>GHMSKSDYIQNMFQTKSFVDRYKYTEKLTGLYAQTLVDYSGVANTSQKPLIVLDNACGIGAVSSVLNHTLQDEAKKTWKLTCGDLSEGMLETTKRRLQDEGWVNAETKIVNALDTGLPDGHYTHVFVAFGFQSFPDANAALKECFRILASGGILASSTWQNFNWIPIMKAAIETIPGNLPFPTQKEFIALHNAGWDSESYIQSELEKLGFRDVKVIPVPKETSIPIDEFFEVCMMIIPYLLPKFWTEEQRESHEKDVPMVLRQYLQDTYGANGQVPLEAVALITTGLKP[2x]

We and others have shown that A. fumigatus effects dithiol gliotoxin S-methylation via a methyltransferase, gliotoxin thiomethyltransferase A (GtmA or TmtA) located outside the gliotoxin gene cluster. GtmA consists of two domains, a larger ‘upper’ domain containing a Rossmann-fold involved in binding the co-substrate SAM and a smaller ‘lower’ domain that changes its relative position to the upper domain in the three crystal structures described here. apo-GtmA seems to be highly flexible, as indicated by the higher B-factors. In agreement with Duell et al., who have recently published the structure of a GtmA–SAH complex in the same crystal form as described here, the cofactor binding site of GtmA is located in the upper part of a cleft between the two domains built by helix α1, sheet β2 and loop regions connecting β1–α2 and β3–β4. Our data suggest that GtmA methylates dithiol gliotoxin by a non-processive mechanism.

According to PDBePISA, the SAH-complexed GtmA forms a stable dimer, as indicated by a buried surface area of 3450 Å2 of 22 640 Å2 total surface area and a solvation free energy gain of −81.3 kcal mol−1. Furthermore, the dimeric arrangement of the SAH complex was not observed in the apo- or SAM-complexed structure, where dimeric arrangements are established via different interfaces. Therefore, the dimer found in the SAH complex is probably a crystallization artefact. The carboxylate group of SAH is hydrogen bonded to Thr27 and Tyr20, residues located in helix α1. The adenyl component of the cofactor is bound to Asn109, the amino group interacts with the backbone carbonyl atom of Ala54, and the ribose hydroxyl moiety is fixed by Asp82. The GtmA–SAH structure reveals a well-shaped hydrophobic cavity close to SAH, which probably represents the binding pocket. Residues Met10, Phe11, Ser131, His189, Tyr237 and Lys241 restrict access to the active site in this structure. However, a combination of our structural and RP-HPLC assay data strongly suggests that GtmA releases MmGT before proceeding to the second methylation step. This seems required, because access to the active site is restricted for both gliotoxin and SAH in the GtmA–SAH structure, suggesting that the binding pocket must be disrupted following the first methyltransfer to release MmGT. No significant difference in BmGT production was noted in samples containing SAH or control samples as detected by RP-HPLC. These results suggest that GtmA was resistant to SAH-mediated feedback inhibition, indicating a low affinity of GtmA towards SAH.>[41x]MRINHNIAALNTLNRLSSNNSASQKNMEKLSSGLRINRAGDDAAGLAISEKMRGQIRGLEMASKNSQDGISLIQTAEGALTETHAILQRVRELVVQAGNTGTQDKATDLQSIQDEISALTDEIDGISNRTEFNGKKLLDGTYKVDTATPANQKNLVFQIGANATQQISVNIEDMGADALGIKEADGSIAALHSVNDLDVTKFADNAADCADIGFDAQLKVVDEAIYQVSSQRAKLGAVQNRLEHTINNLSASGENLTAAESRIRDVDMAKEMSEFTKNNILSQASQAMLAQANQQPQNVLQLLR

There are three parts to the flagellar structure: the trans-membrane basal body that functions as the motor, the connecting rod and hook, and the flagellar filament that acts like a helical propeller. Our current understanding of supercoiling in bacterial flagellar filaments, referred to as polymorphic switching, is based upon the notion that protofilaments within the flagellar filament can exist in two discrete states, that differ slightly in length. The “short” state results from a protofilament having a right-handed inclination (the R-state), while the “long” state results from a protofilament having a left-handed inclination (the L-state). To reconstruct filaments at high resolution, all protofilaments must be “locked” into the same state, either L- or R-type, producing straightened filaments that lead to non-motile bacteria.

While the three L-type mutants (E115G, S285P, and S17P) have a left-handed 11-start helix, the four R-type mutants (N226Y, A233V, H84R and A39VN133H) have a right-handed 11-start helix, and the designations L and R correspond to the hand of these 11-start helices. The L-type 11-start helices are tilted left by ~ 1.7° and the R-type 11-start helices are tilted right by ~ 3.9°. The residue N226 in B. subtilis is not a conserved site and does not form any conserved interactions with other subunits. In the R-type N226Y mutant, the side chain of Y226 in subunit S+5 forms new hydrogen bonds with the side chain of Q110 and the main chain of T107 in subunit S0. But in the L-type subunits, Y226 likely causes major steric clashes. Therefore, N226Y filaments adopt a right-handed form.>[2x]HHHHHHGGAMNIQALLSEKVRQAMIAAGAPADCEPQVRQSAKVQFGDYQANGMMAVAKKLGMAPRQLAEQVLTHLDLNGIASKVEIAGPGFINIFLDPAFLAEHVQQA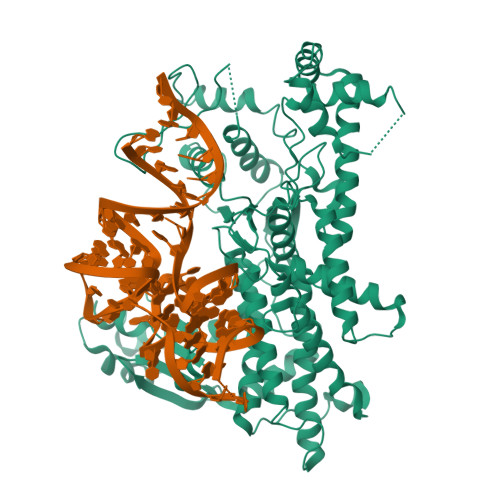LASDRLGVATPEKQTIVVDYSAPNVAKEMHVGHLRSTIIGDAAVRTLEFLGHKVIRANHVGDWGTQFGMLIAWLEKQQQENAGEMELADLEGFYRDAKKHYDEDEEFAERARNYVVKLQSGDEYFREMWRKLVDITMTQNQITYDRLNVTLTRDDVMGESLYNPMLPGIVADLKAKGLAVESEGATVVFLDEFKNKEGEPMGVIIQKKDGGYLYTTTDIACAKYRYETLHADRVLYYIDSRQHQHLMQAWAIVRKAGYVPESVPLEHHMFGMMLGKDGKPFKTRAGGTVKLADLLDEALERARRLVAEKNPDMPADELEKLANAVGIGAVKYADLSKNRTTDYIFDWDNMLAFEGNTAPYMQYAYTRVLSVFRKAEIDEEQLAAAPVIIREDREAQLAARLLQFEETLTVVAREGTPHVMCAYLYDLAGLFSGFYEHCPILSAENEEVRNSRLKLAQLTAKTLKLGLDTLGIETVERM> ETGSAQQLNEDLRLHLLLNTSVTCNDGSPAGYYLKESRGSRRWLLFLEGGWYCFNRENCDSRYDTMRRLMSSRDWPRTRTGTGILSSQPEENPYWWNANMVFIPYCSSDVWSGASSKSEKNEYAFMGALIIQEVVRELLGRGLSGAKVLLLAGSSAGGTGVLLNVDRVAEQLEKLGYPAIQVRGLADSGWFLDNKQYRHTDCVDTITCAPTEAIRRGIRYWNGVVPERCRRQFQEGEEWNCFFGYKVYPTLRSPVFVVQWLFDEAQLTVDNVHLTGQPVQEGLRLYIQNLGRELRHTLKDVPASFAPACLSHEII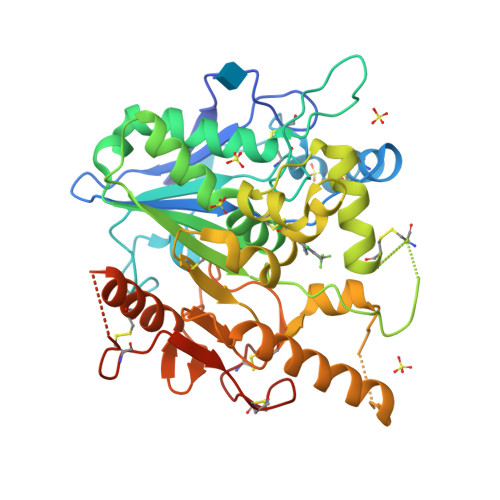IRSHWTDVQVKGTSLPRALHCWDRSLHDSHKASKTPLKGCPVHLVDSCPWPHCNPSCPTGTKHHHHHH>AGTTLTVDLSTTYQRIDGFGTSEAFQRAVQMSRLPEEGQRRALDVLFSTTNGAGLSILRNGIGSSPDMSSDHMVSIAPKSPGSPNNPLIYSWDGSDNKQLWVSQEAVHTYGVKTIYADAWSAPGYMKTNGNDANGGTLCGLSGAQCASGDWRQAYADYLTKYVEFYQESNVTVTHLGFINAPELTTSYASMRFSASQAAEFIRILYPTIQKSNLTYKPTIACCDAEGWNSQAGMLGALSSVNSMFGLVTAHAYTSQPGFSMNTPHPVW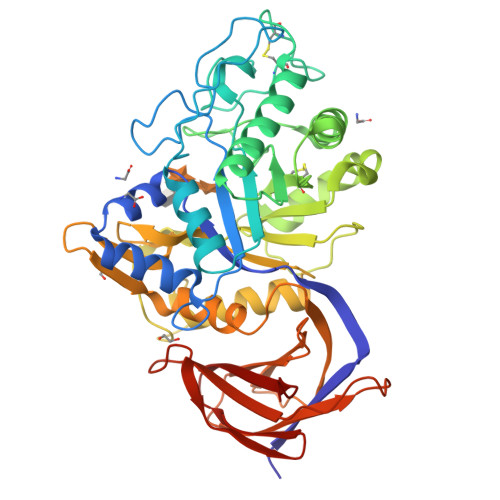MTEAADLQGAWTSAWYSYGGAGEGWTWANNVYNAIVNGNASAYLYWIGAQTGNTNSHMVHIDANAGTVEPSKRLWALGQWSRFVRPGARRVAVSGASGSLRTAAFRNEDGSVAVVVINSGGDAAVNVRLASSSSADQQPASAKAWATDNSRAIEEIQASFADGVATVNVPSRSMTTVVLYPAAD[2x]>MQTSARNQWFGTITARDHDDVQQHVDVLLADGKTRLKVAITAQSGARLGLDEGKEVLILLKAPWVGITQDEAVAQNADNQLPGIISHIERGAEQCEVLMALPDGQTLCATVPVNEATSLQQGQNVTAYFNADSVIIA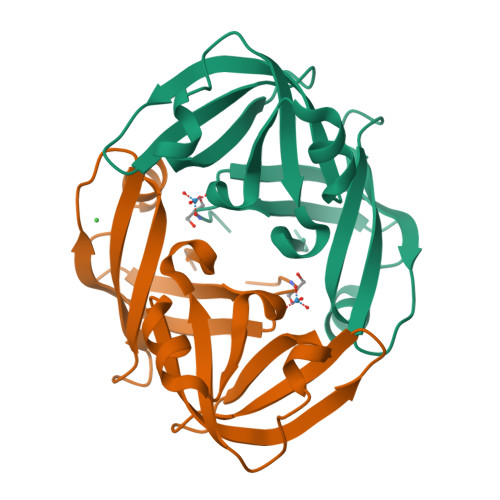TLC[2x]>[3x]GMMNTPESRLVAAGLELPEVAAALGNYEPYSI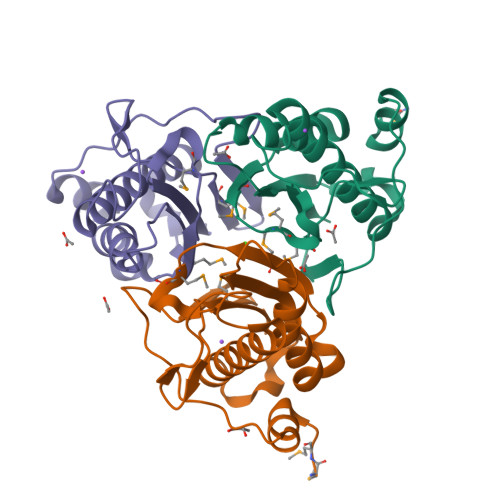VGSQLMTSGQFPYLQGKLLYQGQLGADYTVSEGYAACRLATLNAIAQLKQACGELSRIKQIYRLEGVLNVHQSCIEHPKALDGASDLLLEIFGEAGRHSRMIWTNPVMPLNSLCLVYLFAEL>MDSSISISAIGNVDSPMIRITFQNQTEREFFLNKITDKAKSLGVNISTHPFEIKEPNMVLIKPSKYPDNKLGCYISKNKEIAINFGRTDFRDFVLSNLGVGSHLGTCPTKNETGNDTFYFHQENLSLNGPALSVNTKITKEIEKNDYLLSANGSKAIDFVWSNFLKHPYNPKLKQPDANVKAAWEKHADWEHWSNMGQDWSLNTPSGLVPRPNHGIAHTLRVAQLVPVIAEFLKAYSGDPKFQKLTQKEIQKAQYMMLFSVIGRENDMSWTDANHYQQAFKEAYNGQYSK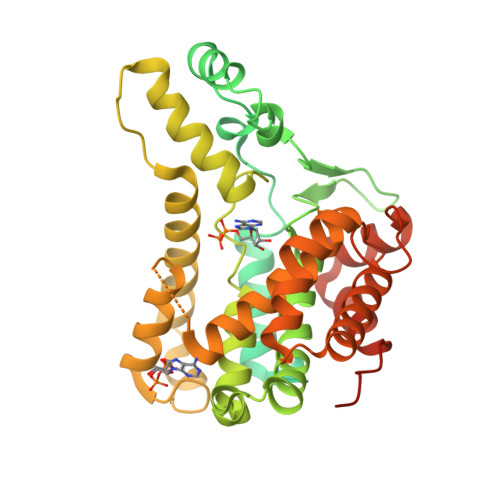HIYATFKENAQKGFLNHVVTNKSSLIPSLFSDESELQYWAEALDTGKPGISSASGILMALAHDLDLMRCYDKGKFNSLKMKDLVARLGGNEDAAKKLADYAHDLIVATGDRCMGYGVTQDYNYSLFGKCSLDPNECLKQLQSIPKPETTLANQYGILEHHHHHH[4x]AcrIIA15 is an anti-CRISPR (Acr) protein that inhibits Staphylococcus aureus Cas9 (SaCas9). The AcrIIA15 protein, consisting of 170 amino acids, is comprised of two domains: an N-terminal domain (NTD) from residues 1 to 56, which contains a HTH motif resembling a transcriptional repressor, and a C-terminal domain (CTD) from residues 57 to 170. AcrIIA15, by combining the HTH domain and Cas9 inhibitory domain within a single protein, exhibits dual functionality as a bi-functional anti-CRISPR protein capable of both transcriptional repression and CRISPR-based cleavage inhibition. Our structural and biochemical studies demonstrate that AcrIIA15 functions as a dimer to simultaneously inhibit both anti-CRISPR operon transcription and SaCas9-sgRNA DNA recognition.

The bending of dsDNA upon binding to AcrIIA15 prompted us to investigate whether AcrIIA15 undergoes conformational changes upon binding promoter DNA. To address this question, we obtained the crystal structure of free AcrIIA15 at a resolution of 2.34 Å. We find that full-length AcrIIA15 exists as a dimer, similar to how it binds to DNA. Notably, the NTDs and the CTDs within the dimer share similar structures to what we observed in the DNA-bound and Cas9-bound structures, respectively. However, due to the different relative positions of the CTD and NTD structural domains in the two monomers, the structures of the two monomers in the same dimer are different. Structural superposition of the AcrIIA15 structures in the free and DNA-bound states showed that they have similar structures, suggesting that DNA binding does not induce significant structural rearrangement in AcrIIA15. The crystal structure and biochemical assays in solution reveal that the full-length AcrIIA15 adopts a dimeric form, while its CTD alone remains as a monomer in solution. The main dimer interface is formed by the loop connecting helices 3 and 4 within the HTH domain, which involves multiple hydrogen bonds and hydrophobic interactions. A hydrophobic core is composed of specific amino acids, namely L44, I5, L8, L9, L32, L39, L42, and L50, from both monomers. Additionally, helix α1 contributes to dimer formation, with residue R2 from one monomer establishing hydrogen bonds with the sidechains of N45 and E48 from the opposite monomer.

>SMRKTIERLLNSELSSNSIAVRTGVSQAVISKLRNGKKELGNLTLNSAEKLFEYQKEMEKVDTWIVYRGRTADMNKSYIAEGSTYEEVYNNFVDKYGYDVLDEDIYEIQLLKKNGENLDDYDVDSDGINNYDKLDEFRESDYVDLEDYDYRELFENSSSQVYYHEFEITHE[4x]Coproporphyrin ferrochelatase (CpfC) in the CPD heme biosynthesis pathway incorporates ferrous iron into coproporphyrin III (cpIII) to give coproheme, which is eventually decarboxylated to yield heme b by the coproheme decarboxylase enzyme in the final step of this biosynthetic process (Dailey et al., 2017; Dailey & Gerdes, 2015; Layer, 2021). Understanding structure–function relationships of key enzymes, such as ferrochelatase, is an essential precondition for the design of new inhibitors for antibiotic‐resistant pathogens, like Listeria monocytogenes. LmCpfC crystals in complex with cpIII were soaked with a ferrous iron solution and flash‐vitrified after 2, 3, and 4 min, to obtain snapshots of the enzymatic reaction during iron insertion into the porphyrin macrocycle. We report three crystal structures showing different iron content during metalation in LmCpfC, identifying the presence and defining the extent of the porphyrin distortions during iron insertion.

Best statistics were obtained when the ferrous iron was placed into the density with an occupancy of 24%. Ring A with the substituent p2 exhibits the highest distortion in the “34% Fe” structure (+12.6°), +9.2° in the cpIII structure and lowered values for the “24% Fe” (+4.8°), and the “68% Fe” (+1.9°) structures; in ring B (p4) the angle is altered the most in the analyzed samples (−13.4°, −10.5°, −11.4°, and −6.7°) as a function of the site occupancy by Fe ions, exhibiting a high degree of distortion compared to the coproheme structure. The measured change of angles throughout the ferrous iron insertion process at the site of p7 at pyrrole ring D is also peculiar: the rings in the substrate‐ and product‐bound states overlap well for all structures besides the “24% Fe” structure (−2.1° in the cpIII‐structure, −1.6° in the "68% Fe" structure, and −1.4° in the "34% Fe" structure). Interestingly, in the “24% Fe” structure ring D is significantly more tilted (−4.2°). In the “24% iron occupancy” and in the coproheme‐bound structures, the guanidinium group points toward p7, while in the “68% iron occupancy” structure, being in a split conformation, partially points outwards since one conformation is 5.4 Å from p7. The residue points toward p7 in the “24% Fe”, “34% Fe”, and in the coproheme‐complex structures, but points away (5.4 Å) in the “68% Fe” structure. Nevertheless, a definitive conclusion cannot be drawn as the ionic radius of the ferrous iron in the “24% Fe”, “34% Fe”, and “68% Fe” structures is larger than the ionic radius of the ferric ion in the coproheme product and would result in an out‐of‐plane position regardless of the side from which it is approaching.

> MTKKVGLLVMAYGTPYKDEDIERYYTDIRHGHKPSEEMIADLRGRYHAIGGLSPLAKITEAQAYGLEKALNDSQDEVEFKAYIGLKHIEPFIEDAVEAMHKDGIEEAISIVLAPHYSSFSVEAYNKRAKEAADKLGGPRINAINDWYKQPKFIQMWADRINETAKQIPADELLDTVLIVSAHSLPEKIKQHNDPYPNQLQETADFIFEKVVVPHYALGWQSEGKTGEPWLGPDVQDLTRELYGREKYKHFIYTPVGFVAEHLEVLYDNDYECKVVTDEVGAAYHRPPMPNSDPEFLEVLRTVVWEKYSNLE> HHHHHHDYKDDDDKADPVPTSKPTPTGKGCHIGRFKSLSPQELASFKKARDALEESLKLKNWSCSSPVFPGNWDLRLLQVRERPVALEAELALTLKVLEAAAGPALEDVLDQPLHTLHHILSQLQACIQPQPTAGPRPRGR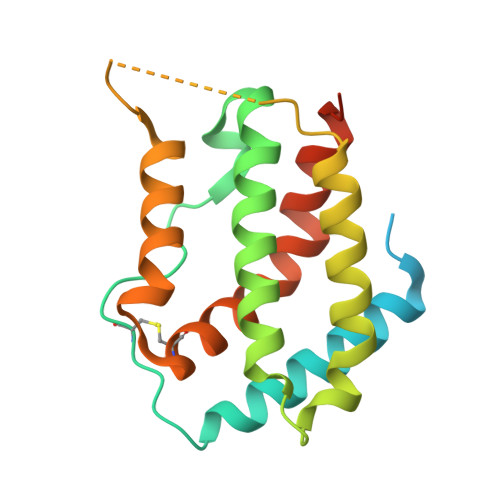LHHWLHRLQEAPKKESAGCLEASVTFNLFRLLTRDLKYVADGNLCLRTSTHPEST> MENDMKSLSAAAQACVKKMRDAKVNEACIRTFIAQHVMVSKGETGSIPDSAIMPVDSLDALDSLTIECDNAVLQSTVVLKLNGGLGTGM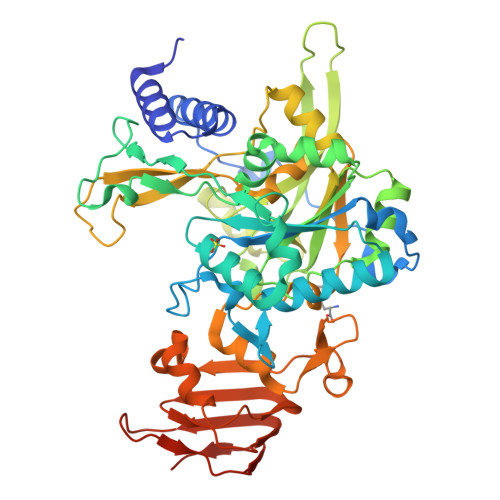GLCDAKTLLEVKDGKTFLDFTALQVQYLRQHCSEHLRFMLMDSFNTSASTKSFLKARYPWLYQVFDSEVELMQNQVPKILQDTLEPAAWAENPAYEWAPPGHGDIYTALYGSGKLQELVEQGYRYMFVSNGDNLGATIDKRVLAYMEKEKIDFLMEVCRRTESDKKGGHLARQTVYVKGKDGQPDAEKRVLLLRESAQCPKADMESFQDINKYSFFNTNNLWIRLPVLLETMQEHGGTLPLPVIRNEKTVDSSNSASPKVYQLETAMGAAIAMFESASAIVVPRSRFAPVKTCADLLALRSDAYVVTDDFRLVLDDRCHGHPPVVDLDSAHYKMMNGFEKLVQHGVPSLVECKRVTVKGLVQFGAGNVLTGTVTIENTDSASAFVIPDGAKLNDTTASPQQSTNKMRPLEHHHHHH> MSGSGSFEGGVFSPYLTGRLPSWAGVRQNVMGSTVDGRPVQPANSSTLTYATLSSSSVDAAAAAAAASAASAVRGMAMGAGYYGTLVANSSSTNNPASLNEEKLLLLMAQLEALTQRLGELTQQVAQLQEQTRAAVA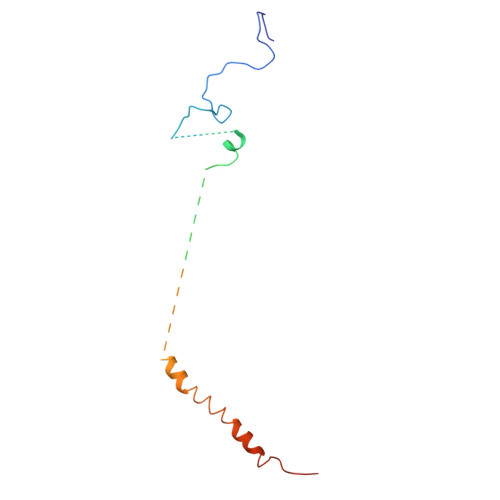TVKSK4-METHYL-PENTANOIC ACID {1-[4-GUANIDINO-1-(THIAZOLE-2-CARBONYL)-BUTYLCARBAMOYL]-2-METHYL-PROPYL}-AMIDE 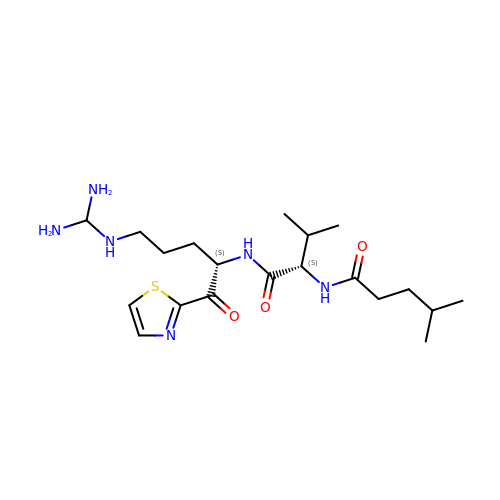| C20 H36 N6 O3 S | ZXELQWLUDMEUHS-HOCLYGCPSA-N> GAMGSTSLEPTSTLVRVRK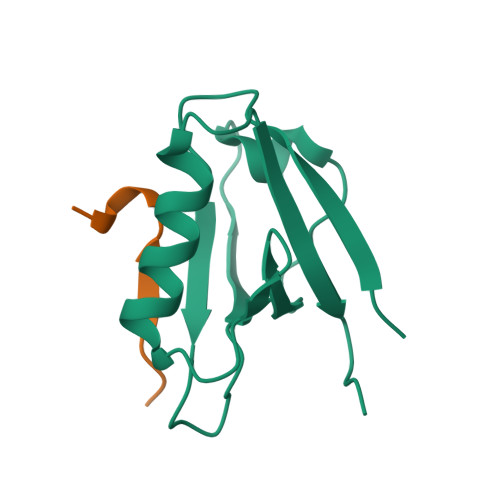SAATLGIAIEGGANTRQPLPRIVTIQRGGSAHNCGQLKVGHVILEVNGQTLRGKEHKEAARIIAEAFKTKERDYIDFLVTEFNVML;> GLPVTFIDEVDSEEAPQ>[2x]GSHMYAS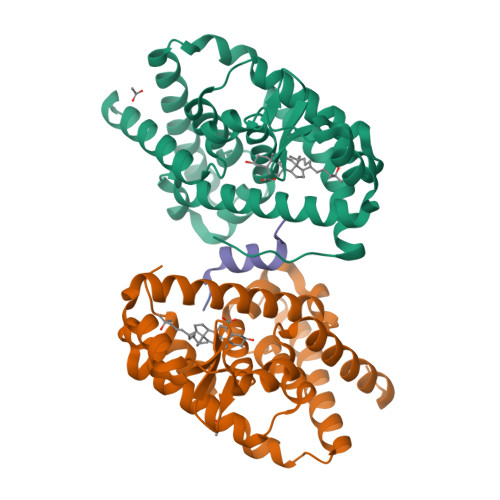LTEIEHLVQSVCKSYRETCQLRLEDLLRQRSNIFSREEVTGYQRKSMWEMWERCAHHLTEAIQYVVEFAKRLSGFMELCQNDQIVLLKAGAMEVVLVRMCRAYNADNRTVFFEGKYGGMELFRALGCSELISSIFDFSHSLSALHFSEDEIALYTALVLINAHRPGLQEKRKVEQLQYNLELAFHHHLCKTHRQSILAKLPPKGKLRSLCSQHVERLQIFQHLHPIVVQAAFPPLYKELFSTETESPVGLSK;> HVERLQIFQHLHPIV>MTQESLLLLDRIDSDDSYASLRNDQEFWEPLARRALEELGLPVPPVLRVPGESTNPVLVGEPGPVIKLFGEHWCGPESLASESEAYAVLADAPVPVPRLLGRGELRPGTGAWPWPYLVMSRMTGTTWRSAMDGTTDRNALLALARELGRVLGRLHRVPLTGNTVLTPHSEVFPELLRERRAATVEDHRGWGYLSPRLLDRLEDWLPDVDTLLAGREPRF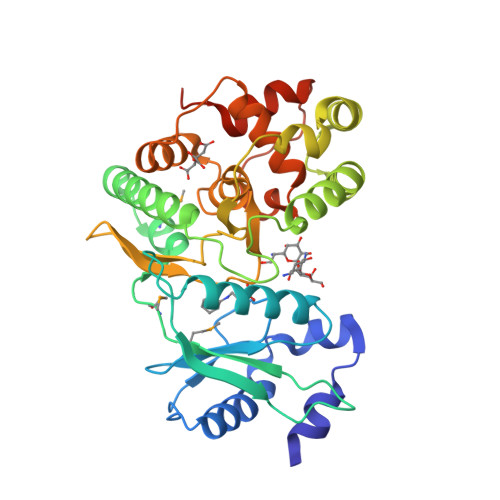VHGDLHGTNIFVDLAATEVTGIVDFTDVYAGDSRYSLVQLHLNAFRGDREILAALLDGAQWKRTEDFARELLAFTFLHDFEVFEETPLDLSGFTDPEELAQFLWGPPDTAPGALEHHHHHH[2x]~{N}-(1-adamantyl)-2-selanyl-benzamide 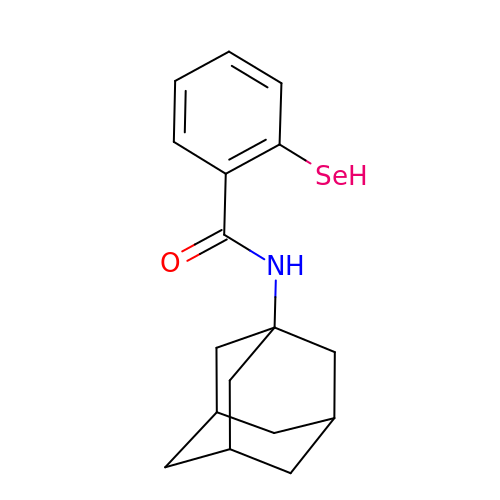| C17 H21 N O Se | CBUMZOCCFOYBIQ-FBBPANFNSA-N Far-red light photoacclimation, or FaRLiP, is a facultative response exhibited by some cyanobacteria that allows them to absorb and utilize lower energy light (700–800 nm) than the wavelengths typically used for oxygenic photosynthesis (400–700 nm). To address these issues, we have isolated a FRL-absorbing PBP complex from cells of the marine cyanobacterium Synechococcus 7335 grown in FRL and solved its structure to a global resolution of 2.78 Å by single-particle, cryo-EM. The fraction containing the FaRLiP-AP core complexes also contained ribulose 1,5-bisphosphate carboxylase oxygenase (Rubisco), and the structure of this enzyme was solved to a global resolution of 2.35 Å.

The FaRLiP-AP core structure was solved to a global resolution of 2.78 Å based on the map-to-map Fourier Shell Correlation, although some map regions were challenging to model due to preferential orientation (see Experimental procedures). It is generally shaped like a cylinder, ∼85 Å in length and ∼95 Å in diameter. Nineteen subunits were identified: eight ApcB2 (β-type subunit), six ApcD5 (α-type subunit), one ApcE2 (α-type subunit with two REP domains (Pfam00427)), one ApcD3 (α-type subunit), one ApcD2 (α-type subunit), one ApcF (β-type subunit), and one ApcC (core linker). Other than the ApcC subunit, which is a core linker protein that assembles into the opening of a trimeric AP toroid, the subunits are arranged as (αβ) heterodimers that further assemble into three (αβ)3 toroids. Trimer 1 and trimer 2 are closely associated, forming a face-to-face hexamer, and trimer 3 is more separated in a tail-to-tail assembly with the trimer 1-trimer 2 toroid. One anion was identified and tentatively modeled as chloride, and each subunit except ApcC binds a single phycocyanobilin chromophore. All phycocyanobilin chromophores are covalently bound to their respective subunits except those bound to ApcD3 and ApcE2. As previously suggested, these chromophores should contribute the most red-shifted absorbance due to the absence of a thioether bond from a Cys sidechain to the vinylidene moiety on pyrrole ring A, which therefore extends the conjugation system in the chromophore. The chromophores of ApcD3 and ApcE2 therefore likely serve as the terminal emitters in the core complex, linking the other phycocyanobilins in the FaRLiP-AP core complex to the Chl molecules in FRL-PSII. Based on all these considerations, we conclude that the FaRLiP-AP core structure determined here is missing one (αβ)3 toroid with an accompanying ApcC subunit.

>[6x]MSLVTELILSADSEARYPAPKELRIFQDFVKTGEQRVRIAKALAANEERIVQNGSQKFWERCPNTPSNSGVDRKTASCQRDQGWYVRLIAYSILAGSERPLEDIGTVGIKEMYNNLEIPIRNIAECMRCLKEEAMAVLSDEDAQEVAAYFDLIIQSLS;>MQDAITTLINTSDAQGKYLDDSSLDTLQEYFRSGDLRAKAAMTISANASTIVTKTVAKSLLYTDITGPGGNMYTCRRYAACIRDMDFFLRYGTYAMLAGDASILDERVLNGLKETYNSLGVPVGATIRAVQAMKEVVNDMLGAEAGKEVGYYFDHICSGLS[8x];> MSIVKQIISNADEELRYPTPGELEMIRSFCKTGASQIQLAKTLESHAPTIVERGTRKFWQICPRTPSNSGSPRKTEAAQRDMSWYIRLISYCLLAGNDQPLREIGLLGMKELYTNIGIPLDNILQYLRCLKAEAIALLSEAEAEAIIPYFDQIIQELVRPGPSYFGIKDRSARQSARQAAA;> MSVISQVIATADREVRYLSKGELDAINRFFNNGPQRLRIVSILNSNAEEIVEKGARRFWQRCPITPSNSDNQQFQASCLRDQAWFIRLISYAVAVGDVDPLEASGVRGVREMYLSLEVPLRSVALCMRSLKEVTLAMLSREDAAEVGPYFDYLIAGLMP;> MRDTVTSLISNYDTTGRYLDRDAIDSLQSYFITGANRVKVAAMISANAAEISREAGKKLFEVVPELIRPGGNAYTTRRYAACLRDMDYYLRYSSYALVAGNNDVLMERVLQGLRETYNSLGVPIAPTVQGIQIMKEMVKERASDMGVDDTSFIDQPFDFISREVSEISV;> MTDRTNGGSPVVHPQQYHTVPTAVINGAHQRDRYPNHSEMQTLSTFLRTGLQRLEIAQTLAQHANEIVAAGGKRIFVGGNPMAYFEQPEELVGMPGSGYFVAEDYLSPKSRRQTGNGHSVQNSSSSITNPVAWLKGLFFSGKPSVPSRFQAINIADYGAVRMKRSMRDLGWFLRYITYAVVAGDTSIITVNTRGLRGIIPEDVTVATTVALQEMQWKSLSFFPVDSAAAALVRRYFDVLIADYQVEKPSDRYRTGVSKHDQGLSFPESYEDSGCAIPRWVMKPTLPDSEKDAVIRAAYRQVFERDISGLGTAELTQPISQLKGEDGSMELFIRQLGKSRLYRQLFYEPYMISRSIELACRHFLGRGLSCMEEFQRYFELVADQGFSALVDALVSSQEYADYFGAETVPYIRGLGIEAQACRNWGPQLDLFKYSAPARKVPQFVTAFASYRQPLPNQHPYGMGNDPLETQFGAIFPHETTNPAAQPVHFSEDSRRILVGHAHRKSHAEISQQIFSLKTLAHKPTKASESLSFFPSSDSRQHSVESVILAAYRQVFGCEVLGSQRHQAAETQLKGGLITVREFVRQLAKSRSFRQAYWENLYMTKAAEIIHRRLLGRPTYGRRETSKYYDICGRQGFYALVDALIDSDDYRTAFGENTVPYERYVTPRGLALRSPKGPVAISKLRDNPHTVGEYMMRYQPPAANISPRSPLNNSASNRQPATARHSDNGALEDRSASSTEPATSKSSVALADPPASDEPAASEDSAISENIEPSMAVALQETSSD;> MRMFRVTACVPSQTRIRTQRELQNTYFTKLVPYDNWFKEQQRIQKMGGTIVKVELATGRRGANTGLA>[2x]MEYGKKVNYQQFDNIYLGAEASVVSCFLQDSEGLIWIGSNKGLFSYDGYSTQQHFTYGENNNTRIYCGVIIDNTYLYMGTDNGILVYNYRADRYEQPETDFPTDVRTMALQGDTLWLGALNGLYTYQLQSRKLTSFDTRRNGLPNNTIYSIIRTKDNQIYVGTYNGLCRYIPSNGKFEGIPLPVHSSQSNLFVNSLLEDTTRQCVWIGTEGYLFQYFPSTGQIKQTEAFHNNSIKSLALDGNGDLLAGTDNGLYVYHNDTTPLQHIIHDSRNIQSLTNNIIWNIFADQEHNIWLGTDYGISLSRYNSALQFIPISQITGTGDGNQFYSLFRDSKGFYWFGGANGLIRFTDPAGERHDAIWYRMGDKTYPLS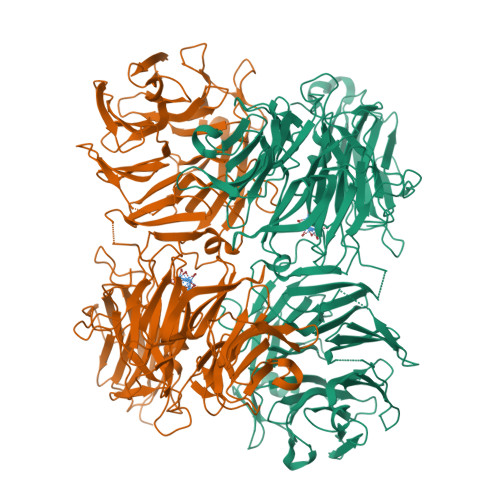HNRIRHIYEDKEQQLWIATDGSINRYDYATRQFIHYNIVDNTGTYNTNWTYYIFEDTAGQLWISTCLGGIFVVDKHKLMQSTSGQYIAEQNYSVHNGLSGMFINQIIPDNEGNVWVLLYNNKGIDKINPRTREVTKLFADELTGEKSPNYLLCDEDGLLWVGFHGGVMRINPKDESQQSISFGSFSNNEILSMTCVKNSIWVSTTNGLWIIDRKTMDARQQNMTNKRFTSLLFDPKEDCVYLGGADGFGISHSNLEATYQPERPILLTALYINNQLVSPRTRDDVPNIRYTNSIKLKYDQNNLSFELSDLPYSLDEKNKFVYRLEGMDKEWNFLKSNINRITYSNLSYGNYQLIISKLERDGQPSNRPHILNIRILPPWLEHHHHHH4-(benzylamino)-6-({4-[(1-methylpiperidin-4-yl)carbamoyl]phenyl}amino)pyridine-3-carboxamide 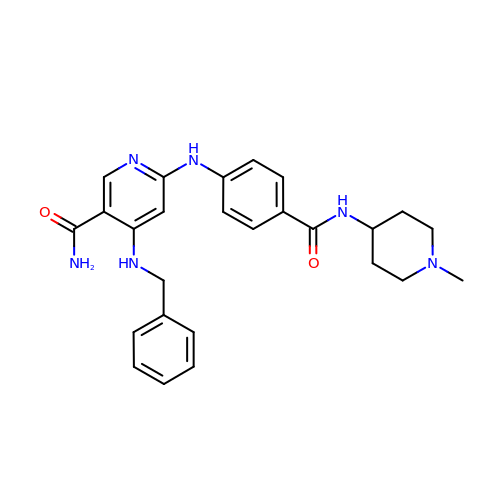| C26 H30 N6 O2 | NYSLPKXXILEKDL-UHFFFAOYSA-N> MALTTTGTEQHDLFSGTFWQNPHPAYAALRAEDPVRKLALPDGPVWLLTRYADVREAFVDPRLSKDWRHTLPEDQRADMPATPTPMMILMDPPDHTRLRKLVGRSFAVRRMNELEPRITEIADGLLAGLPTDGPVDLMREYAFQIPVQVICELLGVPAEDRDDFSAWSSVLVDDSPADDKNAAMGKLHGYLSDLLERKRTEPDDALLSSLLAVSDEDGDRLSQEELVAMAMLLLIAGHETTVNLIGNGVLALLTHPDQRKLLAEDPSLISS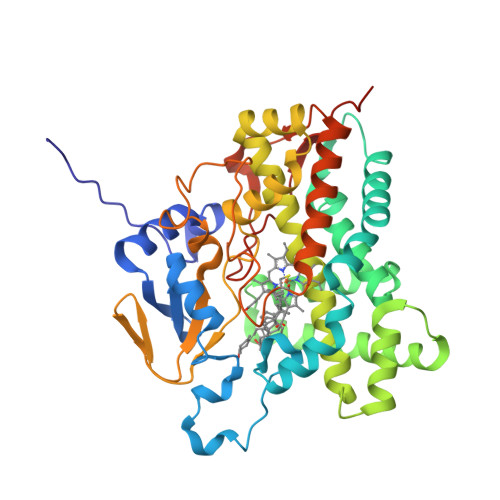AVEEFLRFDSPVSQAPIRFTAEDVTYSGVTIPAGEMVMLGLAAANRDADWMPEPDRLDITRDASGGVFFGHGIHFCLGAQLARLEGRVAIGRLFADRPELALAVGLDELVYRESTLVRGLSRMPVTMGPRSALEHHHHHH> EWGAPETLQRCLEENQELRDAIRQSNQILR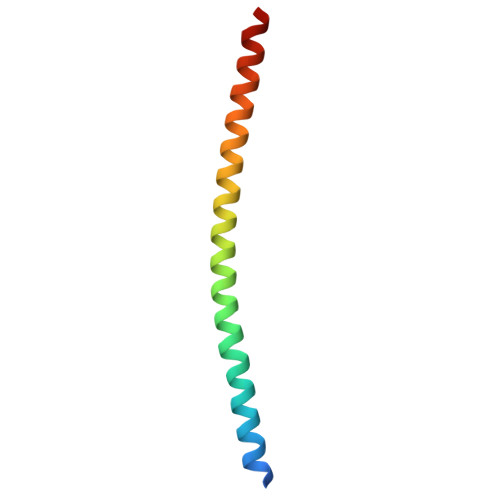ERCEELLHFQASQREEKEFLMCKFQEARKLVERLGLEK>[4x]MRGSHHHHHTTGEDDESECVINYVEKAVNKLTLQMPYQLFIGGEFVDAEGSKTYNTINPTDGSVICQVSLAQVSDVDKAVAAAKEAFENGLWGKINARDRGRLLYRLADVMEQHQEELATIEALDAGAVYTLALKTHVGMSIQTFRYFAGWCDKIQGATIPINQARPNRNLTLTKKEPVGVCGIVIPWNYPLMMLSWKTAACLAAGNTVVIKPAQVTPLTALKFAELTLKAGIPKGVVNILPGSGSLVGQRLSDHPDVRKIGFTGSTEVGKHIMKSCALSNVKKVSLALGGKSPLIIFADCDLNKAVQMGMSSVFFNKGENCIAAGRLFVEESIHNQFVQKVVEEVEKMKIGNPLERDTNHGPQNHEAHLRKLVEYCQRGVKEGATLVCGGNQVPRPGFFFQPT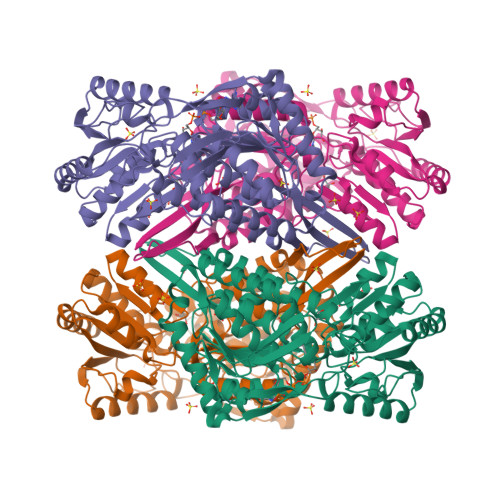VFTDVEDHMYIAKEESFGPIMIISRFADGDVDAVLSRANATEFGLASGVFTRDINKALYVSDKLQAGTVFINTYNKTDVAAPFGGFKQSGFGKDLGEAALNEYLRIKTVTFEY>MGKIVGIIGGMGPVATVKFIEKLTSMTDAEIDQDHVRYVLYNDPEIPDRIEAYFENMESPVNAINNGIKYLESIGIDTIGMACNTAHIWFKEFVYKSNFLNMIDLTASVLKKSGFKNVLLLSTNATVSSGIYTGKLRDYNINTVIPDQDIVMKSIHYVKVNDTKMARETIEPVING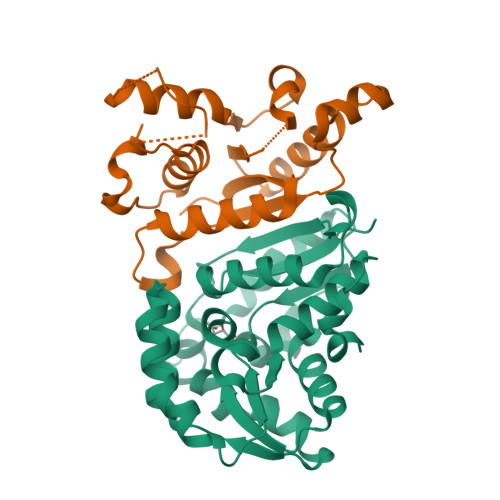HRNEVDALLLACTEMPVIISEKTYNIPVIDSDEALAAALIKSAGKRLKKEYRLYDL[2x]The most relevant are the cysteine peptidases gingipain K (alias Kgp) and R (RgpA and RgpB), which cleave proteins and peptides after lysines and arginines, respectively. Kgp, which is responsible for most of this activity, is a 1723/1732-residue multidomain enzyme encompassing an N-terminal signal peptide, a pro-domain for latency, a caspase-like cysteine peptidase catalytic domain (CD), an immunoglobulin superfamily-like domain (IgSF), between three and five hemagglutinin-adhesion domains, and the C-terminal domain for type-IX secretion. Kgp degrades connective tissue and plasma proteins, for example heme- and hemoglobin-transporting proteins, fibrinogen, fibronectin, plasma kallikrein, immunoglobulins, as well as peptidase inhibitors, thus causing vascular permeability and bleeding. Taken together, these domains form an elongated structure that resembles a tooth: the CD forms the crown with the cusp at its top, and the IgSF, which is a six-stranded antiparallel open β-barrel, shapes the root.

Here, we analyzed the crystal structure of Kgp from P. gingivalis strain W83 in complex with KYT-36 to very high resolution (1.20 Å). KYT-36 is a L-peptide-derived molecule that mimics a substrate binding in extended conformation to cleft sub-sites S3, S2, S1 and S1’. The BOC benzyl group nestles in a hydrophobic pocket created by the side chains of H575 and W391, which together with Y512 and W513 create a shallow S3 sub-site in Kgp. The LYS group of KYT-36 simulates a substrate residue in P1 and thus matches the specificity of the enzyme. Its side chain penetrates the specificity pocket and its aliphatic part is pinched between W513, A451 and C476 through hydrophobic interactions. The terminal ε-amino group is tetrahedrally bound by D516Oδ2 through a salt bridge, by N475O and T442Oγ1 through direct hydrogen bonds, and by Y517N and W513O through hydrogen bonds mediated by a solvent molecule. The carbonyl carbon is just 2.02 Å apart (2.00 Å and 2.03 Å in the two Kgp molecules A and B found in the asymmetric unit of the crystal, respectively) from catalytic C477Sγ, which is roughly perpendicular to the carbon and its three bound atoms. In addition, the inhibitor carbonyl carbon is pyramidalized, i.e. not coplanar with its three bound atoms but shifted towards a tetrahedral configuration. Thus, the present structure simulates a state immediately previous to formation of the tetrahedral reaction intermediate of the nucleophilic addition. The complex structure of Kgp with its specific inhibitor KYT-36 revealed that the sub-nanomolar inhibition exerted by the inhibitor is based on 24 intermolecular interactions and the fact that the active-site cleft of the enzyme is blocked from sub-sites S3 to S1’.

>DVYTDHGDLYNTPVRMLVVAGAKFKEALKPWLTWKAQKGFYLDVHYTDEAEVGTTNASIKAFIHKKYNDGLAASAAPVFLALVGDTDVISGEKGKKTKKVTDLYYSAVDGDYFPEMYTFRMSASSPEELTNIIDKVLMYEKATMPDKSYLEKVLLIAGADYSWNSQVGQPTIKYGMQYYYNQEHGYTDVYNYLKAPYTGCYSHLNTGVSFANYTAHGSETAWADPLLTTSQLKALTNKDKYFLAIGNCCITAQFDYVQPCFGEVITRVKEKGAYAYIGSSPNSYWGEDYYWSVGANAVFGVQPTFEGTSMGSYDATFLEDSYNTVNSIMWAGNLAATHAGNIGNITHIGAHYYWEAYHVLGDGSVMPYRAMPKTNTYTLPASLPQNQASYSIQASAGSYVAISKDGVLYGTGVANASGVATVSMTKQITENGNYDVVITRSNYLPVIKQIQVGEPHHHHHH[2x]> DNQFYSVEVGDSTFTVLKRYQNLKPIGSGAQGIVCAAYDAVLDRNVAIKKLSRPFQNQTHAKRAYRELVLM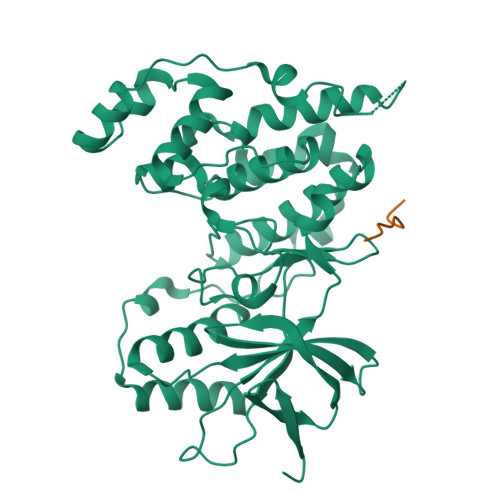KCVNHKNIISLLNVFTPQKTLEEFQDVYLVMELMDANLCQVIQMELDHERMSYLLYQMLCGIKHLHSAGIIHRDLKPSNIVVKSDCTLKILDFGLARTAGTSFMMTPYVVTRYYRAPEVILGMGYKENVDIWSVGCIMGEMVRHKILFPGRDYIDQWNKVIEQLGTPCPEFMKKLQPTVRNYVENRPKYAGLTFPKLFPDSLFPADSEHNKLKASQARDLLSKMLVIDPAKRISVDDALQHPYINVWYDPAEVEAPPPQIYDKQLDEREHTIEEWKELIYKEVMN;> KHEMTLKF Givinostat | 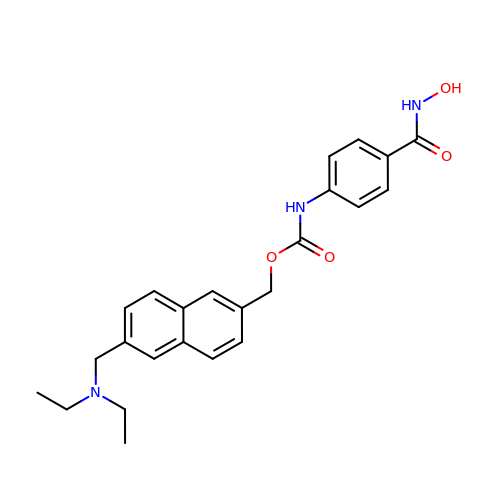C24 H27 N3 O4 | YALNUENQHAQXEA-UHFFFAOYSA-N>[3x]GAMGSLIRKKAAGLESAATIRTKVFVWGLNDKDQLGGLKGSKIKVPSFSETLSALNVVQVAGGSKSLFAVTVEGKVYACGEATNGRLGLGISSGTVPIPRQITALSSYVVKKVAVHSGGRHATALTVDGKVFSWGEGD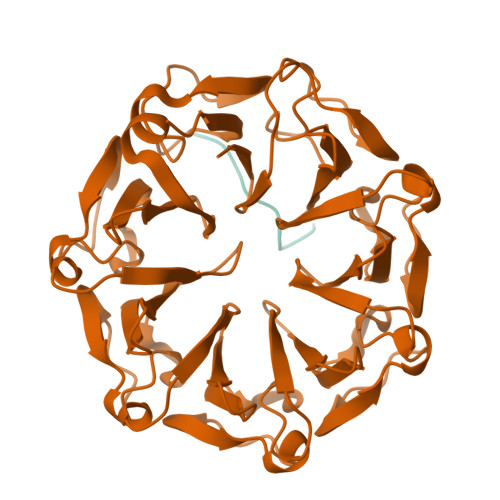DGKLGHFSRMNCDKPRLIEALKTKRIRDIACGSSHSAALTSSGELYTWGLGEYGRLGHGDNTTQLKPKMVKVLLGHRVIQVACGSRDAQTLALTDEGLVFSWGDGDFGKLGRGGSEGCNIPQNIERLNGQGVCQIECGAQFSLALTKSGVVWTWGKGDYFRLGHGSDVHVRKPQVVEGLRGKKIVHVAVGALHCLAVTDSGQVYAWGDNDHGQQGNGTTTVNRKPTLVQGLEGQKITRVACGSSHSVAWTTVDVATPSVHEPVLFQT;>AKDEDKDEDEKEKAA[3x]Bile salt hydrolases (BSHs) comprise a diverse family of microbial enzymes that catalyse critical BA transformation. Primary conjugated BAs synthesized in the liver, such as the tauro- and glycoconjugates of cholic acid (TCA, GCA), are deconjugated by BSHs to generate cholic acid (CA) (BA names and abbreviations are summarized in Supplementary Fig. 1). We found that Lactobacillaceae BSHs display a clear bias for either glycine or taurine-conjugated BAs. Notably, each monomer contains a loop that swaps into the active site of a neighbouring monomer within the tetramer and places amino acids proximal to the catalytic residues.

To examine the molecular foundations of BSH substrate specificity, we determined the crystal structures of six of the Lactobacillaceae BSHs examined above: four glycine-preferring (LgasBSHb, LaciBSHa, LingBSH, LreuBSH) and two taurine-preferring (LgasBSHa, LjohBSHc) BSHs. We examined the sequences of these loops and found that taurine-preferring enzymes exclusively contained G-V/T-G (‘G-X-G’) motifs, while glycine-preferring enzymes solely contained S-R-G/S (‘S-R-X’) motifs. While activity with MCBAs is relatively low compared with conventional BAs, some BSHs such as LingBSH and LreuBSH exhibit appreciable activity. To examine the recalcitrance of MCBAs more broadly, we monitored the deconjugation kinetics of 5 BSHs that had previously exhibited assorted substrate preferences (LingBSH, LgasBSHa, LgasBSHb, LjohBSHc and LreuBSH).

> MCTSVIYTAGDYYFGRNLDLEVNLGQEVVITPRNKTLEFREMPNLEHHYAIIGMSIVRDDYPLYFDGVNEKGVGMAGLNFDGPAHYFPVQEGKDNIASFELVPYILAAASSVAEAKKLLSNANIANINFSDKLQAAPLHWIIADKTGASVTVESTAKGLNVYDNPVGVLTNNPEFPRQLLNLSNYRSVAPANPANVFAPNVDLPVYSRGLGTHFLPGGMDSESRFVKATFTKMHAPVGNSEVENITNYFHILQSVEQQKGLDEVAPNTFEYTIYSDGSNLKKGIFYYKTYENSQINAVDMHKEDLEASELITYPVQNKQIINQQNHHHHHH> ECTPGQTKKQDCNTCTC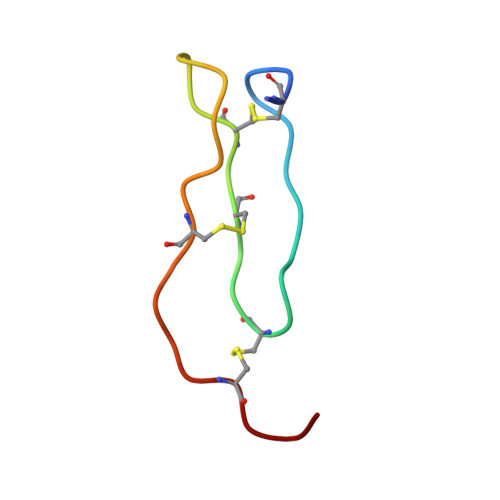TPTGIWGCTRKACRTT>[2x]GPLGSMSVLRPLDKLPGLNTATILLVGTEDALLQQLADSMLKEDCASELKVHLAKSLPLPSSVNRPRIDLIVFVVNLHSKYSLQNTEES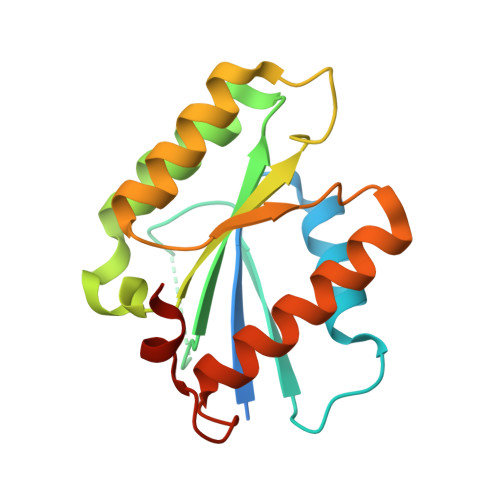LRHVDASFFLGKVCFLATGAGRESHCSIHRHTVVKLAHTYQSPLLYCDLEVEGFRATMAQRLVRVLQICAGHVPGVSALNLLSLLRS>[6x]GAMGSGIQMKEEASEHGGSADETQELSPVSDSSDEMPNNAKRRRRSQSMIANKRIHQAFQEDEGDEDWEEEEHKPKAKRRYNTRSNESFSEGDDEPFEVSESSALEDELSDSEDSFIRSVRSKPKYKPGTRRSTRLRNRRSQDEEESEEEHRPILRERTSRINYSVPLAFPPVDEMDGDPSSQVNQSRSRKTHSELAITKLLRQQVSSFMPYIDSSGSESESDNTRIKKSSAKTIKALTDPANSGGPPDFGRIREKSDLADSDPLGVDSSLSFESVGGLDNYINQLKEMVMLPLLYPEIFQRFNMQPPRGVLFHGPPGTGKTLMARALAAACSSENKKVSFYMRKGADCLSKWVGEAERQLRLLFEEAKSTQPSIIFFDEIDGLAPVRSSKQEQIHASIVSTLLALMDGMESRGQVIIIGATNRPDAVDPALRRPGRFDREFYFPLPDRDARKKIIEIHTRNWDPPVPEWLCSMLAEKSKGYGGADLRALCTEAALNSIKRTYPQLYRSTKRLQIDPKTIKVKVKDFVMSMKRMIPSSERSSISPSKPLSPELKPLLNEAFQDIEKTLQKLMPVASKLNPLEEVMYDDPKENDFEYQQRLETFETLRIYKPRFLICGRKGLG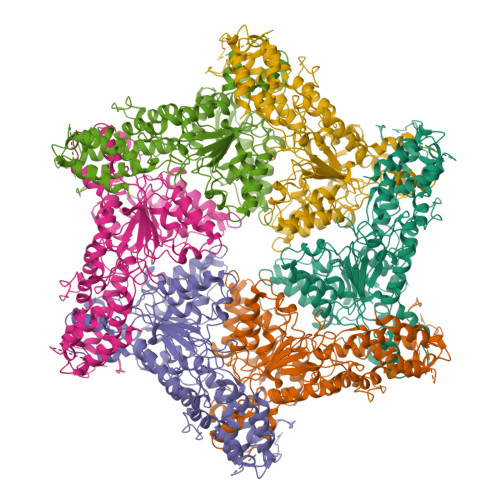QTALGPAILQQYEGVHVQSFDMSTLLQDSTQSIETSIIHLFLEVRRHTPSIIYIPDIDNWLNVLPLTAITTFSSMLERLDFSDQILFLALSSSPLSELHPQLREWFSSKQSVYSLQYPTRDSIIAFFQPILELIKASPTELPGGIPRKRRVLPELPLAPDPPPFTSQKITLKQTKQADMRLLNKLKIKLNALLGSLRARYRKFKKPLIDFNDIYCVDPETGHSYRSREECHYEFVDDVVKQIGSDQKFSMMSLEEIEKRTWDNCYCTPKQFVHDIKLILRDALQLEDSETIKRAQEMYANVLLGVEDMEDDQFSQRCERMALREAERRKLRHGKLQKHLDETKADMQFTSEKPSVDESITEVDDAIKDGPPVLAETLTNSLMEDVGPENVDMDIEDNEIFTNQSTMSVPSMLVENEESPKPDEYIDQKDKVQSPLLNGKSPVGVPSEAALRVSTDVSTNISSNGRADIPVDTLITSPADVPNNAPTDAHNITSADGHIENIEQEVVFPDLVFDEDRLTPLKQLLIDSTTGFTVDQLLHLHSFLYQIIWNTKSEWNRNSVVDECERAVKEFMINALQ>[4x]MPVFTASFQCVTLFGQPASAADAQPLLQGQRPFLHLHARRRRPCGPMLISKSPPYPASEETREWEADGQHEHTDELRETTTTMIDGIRTALRSIGEGEISISAYDTSLVALLKRLDGGDGPQFPSTIDWIVQNQLPDGSWGDASFFMMGDRIMSTLACVVALKSWNIHTDKCERGLLFIQENMWRLAHEEEDWMLVGFEIALPSLLDMAKDLDLDIPYDEPALKAIYAERERKLAKIPRDVLHSMPTTLLHSLEGMVDLDWEKLLKLRCLDGSFHCSPASTATAFQQTGDQKCFEYLDGIVKKFNGGVPCIYPLDVYERLWAVDRLTRLGISRHFTSEIEDCLDYIFRNWTPDGLAHTKNCPVKDIDDTAMGFRLLRLY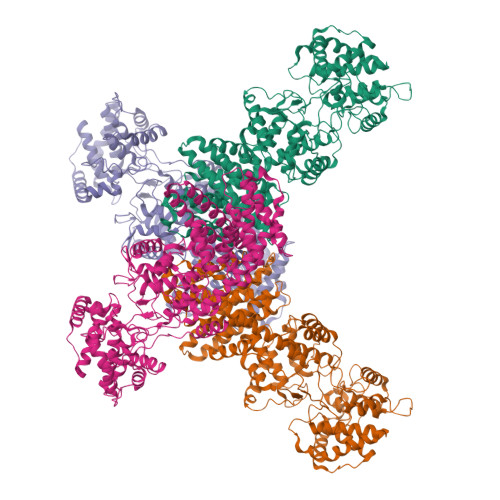GYQVDPCVLKKFEKDGKFFCLHGESNPSSVTPMYNTYRASQLKFPGDDGVLGRAEVFCRSFLQDRRGSNRMKDKWAIAKDIPGEVEYAMDYPWKASLPRIETRLYLDQYGGSGDVWIGKVLHRMTLFCNDLYLKAAKADFSNFQKECRVELNGLRRWYLRSNLEKFGGTDPQTTLMTSYFLASANIFEANRAAERLGWARVALLADAVSSHFRRIGGPKNSTSNLEELISLVPFDDAYSGSLREAWKQWLMAWTAKESSQESIEGDTAILLVRAIEIFGGRHVLTGQRPDLWEYSQLEQLTSSICCKLSRRVLAQENGESTEKVEEIDQQVDLEMQELTRRVLQGCSAINRLTRETFLHVVKSFCYVAYCSPETIDSHIDKVIFQDVIEFHHHHHH>MSLSDLTIQKVESRILDVPLIRPHGFATTTSTEQHILLVSVHLENGVIGYGEGVVPGGPWWGGESVETMKALVDGYLAPVLIGRAVSELAGIMADLERVVARARYAKAAVDVAMHDAWARSLNVPVRDLLGGTVRDKVDVTWALGVLPLDVAVAEIEERIEEFGNRSFKLKMGAGDPAEDTRRVAELAREVGDRVSLRIDINARWDRRTALHYLPILAEAGVELFEQPTPADDLETLREITRRTNVSVMADESVWTPAEALAVVKAQAADVIALKTTKHGGLLESKKIAAIAEAGGLACHGATSLEGPIGTAASLQFAASTKAISYGTELFGPQLLKDTYIVQEFEYKDGQVAIPQGPGLGVDVDMDKVNF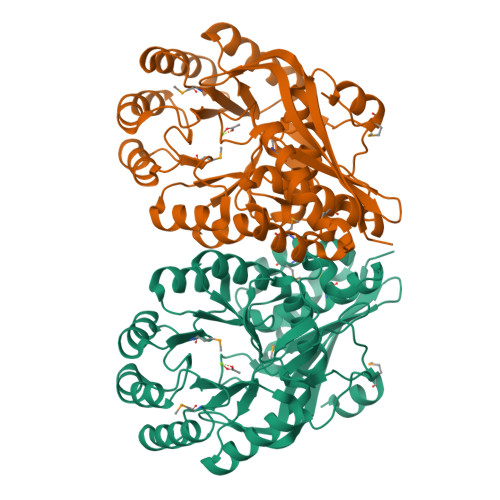YTRKEGHHHHHH[8x]>XGELKAIAQELKAIAK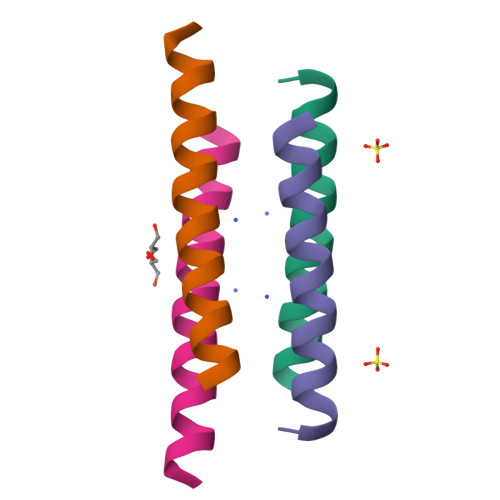ELKAIAWEKKAIAQGX[2x]>MERLVWDKLTLLGFLEKNHIPQKLYYNLSSQDKELSAEIQSNVTYYTLRDANNTLIQALIPISQDLQIHIYKKGEDYFLDFIPIIFTRKEKTLLLSLQTSPYQDIIKATNDPLLANQLMNAYKKSVPFKRLVKNDKIAIVYTRDYRVGQAFGQPTIKMAMVSSRSNQYYLFSHSNGHYYDSKAQEVAGFL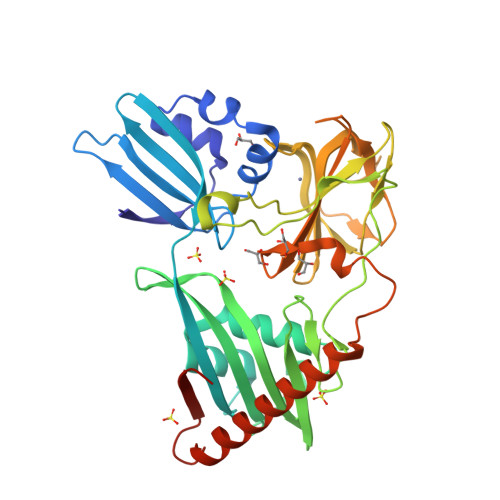LETPVKYTRISSPFSYGRFHPVLKVRRPHYGVDYAAKHGSLIHSASDGRVGFMGVKAGYGKVVEIHLNELRLVYAHMSAFANGLKKGSFVKKGQIIGRVGSTGLSTGPHLHFGVYKNSRPINPLGYIRTAKSKLHGKQREVFLEKAQRSKQKLEELLKTHSFEKNSFYLLEGFLEHHHHHH[2x]> MLKQVEIFTNGSCLGNPGPGGYGAILRYRGREKTFSAGYTRTTNNRMELMAAIVALEALKEHCEVILSTDSQYVRQGITQWIHNW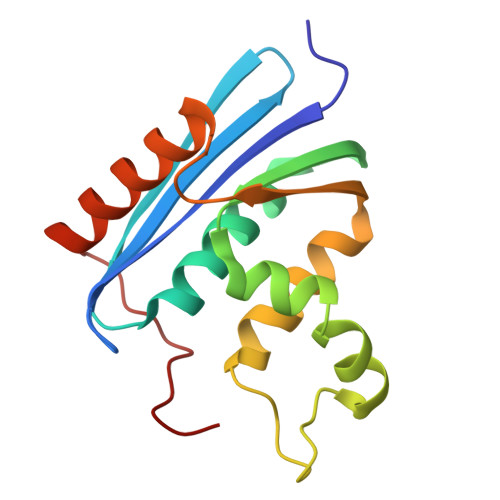KKRGWKTADKKPVKNVDLWQRLDAALGQHQIKWEWVKGHAGHPENERCDELARAAAMNPTLEDTGYQVEV FAM92A1, also named CIBAR1, is a BAR domain protein that functions in important processes involving membrane remodeling, such as mitochondrial crista ultrastructure and ciliogenesis. FAM92A1 preferentially interacts with the negatively charged phospholipids PI(4,5)P2 and cardiolipin to induce extensive membrane curvature. Furthermore, FAM92A1 is predicted to feature a BAR domain at its N-terminus and an unstructured short tail at its C-terminus. By determining the crystal structure of the FAM92A1 BAR domain, combined with atomistic molecular dynamics simulations, we uncover that FAM92A1 interacts with phosphoinositide- and cardiolipin-containing membranes to induce lipid-clustering and membrane curvature.

Thus, to elucidate the structural basis for its membrane remodeling activity, we purified and crystallized the FAM92A1 N-terminal region (residues 1–219). The crystal structure of FAM92A1 BAR domain was solved at 2.03 Å resolution. Based on the crystal structure, the region spanning residues 2–211 was coiled-coil composed of three α helices, designated as the FAM92A1 BAR domain. In the asymmetric unit of the crystals, two FAM92A1 BAR domain monomers assembled via a two-fold symmetric interface, yielding a banana-shaped homo-dimer characteristic for BAR-domain proteins. The BAR domain is finalized by a last long helix (α3) covering amino acids 142–211. In the second chain α2 helix, the loop between α2 and α3 is partially disordered from Lys125 to His142, indicating some flexibility in the structure at the distal ends. The overall dimensions of the dimeric BAR domain are 150 Å in total length and ca. 25 Å in diameter around the center of the six-helical dimer bundle. The dimer interface is extensive with a total interface area of 2532 Å2 involving 65 hydrophobic residues with >70% buried surface area at the interface and 11 hydrogen-bonded interactions across the interface. Specifically, the angle between the α2 helices of the two chains in the FAM92A1 BAR domain is 33.2°, a value that is consistent with other classical BAR domains, including N-BAR domain proteins. Consistently, the membrane interacting residues identified in our previous in vitro lipid-binding assay, including Lys107, Lys109, and Arg110 and Arg132, Arg134, and Arg136, form two positive charged clusters located on the concave surface of the FAM92A1 BAR domain dimer. Furthermore, an analysis of the electrostatic potential surface of the FAM92A1 BAR domain revealed the characteristic accumulation of positive electrostatic potential/charge on the concave surface.

>[2x]MMRRTLENRNAQTKQLQTAVSNVEKHFGELCQIFAAYVRKTARLRDKADLLVNEINAYAATETPHLKLGLMNFADEFAKLQDYRQAEVERLEAKVVEPLKTYGTIVKMKRDDLKATLTARNREAKQLTQLERTRQRNPSDRHVISQAETELQRAAMDASRTSRHLEETINNFERQKMKDIKTIFSEFITIEMLFHGKALEVYTAAYQNIQNIDEDEDLE> PGDPQICPKRCVCQILSPNLATLCAKKGLLFVPPNIDRRTVELRLADNFVTNIKRKDFANMTSLVDLTLSRNTISFITPHAFADLRNLRALHLNSNRLTKITNDMFSGLSNLHHLILNNNQLTLISSTAFDDVFALEELDLSYNNLETIPWDAVEKMVSLHTLSLDHNMIDNIPKGTFSHLHKMTRLDVTSNKLQKLPPDPLFQRAQVLATSGIISPSTFALSFGGNPLHCNCELLWLRRLSREDDLETCASPPLLTGRYFWSIPEEEFLCEPPLITRHTHEMRVLEGQRATLRCKARGDPEPAIHWISPEGKLISNATRSLVYDNGTLDILITTVKDTGAFTCIASNPAGEATQIVDLHIIAAAHHHHHH

SALMs, also known as leucine-rich and fibronectin III domain-containing proteins, are a family of newly characterized SAMs that belong to the type I transmembrane proteins. Members of the SALM family are predominantly expressed in the central nervous system (CNS) and known for their engagement in neurite outgrowth, synapse formation, and synapse maturation. LAR-RPTPs are type I transmembrane proteins and share a common domain architecture of an ectodomain containing up to three immunoglobulin-like (Ig) domains and up to nine fibronectin III (Fn) repeats, followed by a transmembrane domain and tandem intracellular phosphatase domains.

The asymmetric unit of the free SALM5 crystal contained one SALM5 molecule. Except two loops, most residues in the Ig domain of SALM5 were not determined in the free SALM5 crystal due to lack of density, suggesting dynamic movement or multiple conformations of the Ig domain. As demonstrated by crystal packing analysis and structural superimposition, the free and PTPδ-bound SALM5 structures unanimously revealed that two SALM5 molecules form a diad dimer through their LRR domains packing in an antiparallel side-by-side manner. Dimerization of SALM5 is exclusively mediated by its LRR domain. The two protomers in the SALM5 dimer are related by a twofold axis, and the dimer interface buries a total of ~2200 Å2 solvent accessible surface area (SASA) with a long list of residues involved. The LRR domains of two SALM5 molecules constitute a concave platform as the core of the dimer, with approximate dimensions of 56 Å × 68 Å. The SALM5 LRR-Ig totally adopts a totally all-β fold, with the overall structure in an L-shape. The LRR domain resembles a solenoid with its concave side lined with ten long parallel β-strands and convex side comprising variable loops, short β-strands and 310 helical segments. In the site A, two sets of ascending loops in the LRRs 3–6 are intertwined at the dimer interface, and an extensive hydrogen network is built by engagement of residues R110, Q134, and N158. The guanidine group of the residue R110 from one protomer forms four hydrogen bonds with the side chain amide group of N158 and the main chain carbonyl oxygen atoms of N157 and H180 from the other protomer.> MKESYYSIGEVSKLANVSIKALRYYDKIDLFKPAYVDPDTSYRYYTDSQLIHLDLIKSLKYIGTPLEEMKKAQDLEMEELFAFYTEQERQIREKLDFLSALEQTISLVKKRMKRQMEYPALGEVFVLDEEEIRIIQTEAEGIGPENVLNASYSKLKKFIESADGFTNNSYGATFSFQPYTSIDEMTYRHIFTPVLTNKQISSITPDMEITTIPKGRYACIAYNFSPEHYFLNLQKLIKYIADRQLTVVSDVYELII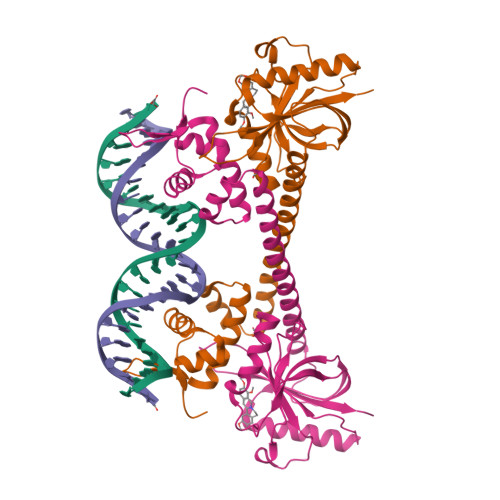PIHYSPKKQEEYRVEMKIEILDHHHHHH> AFVVTDNCIKCKYC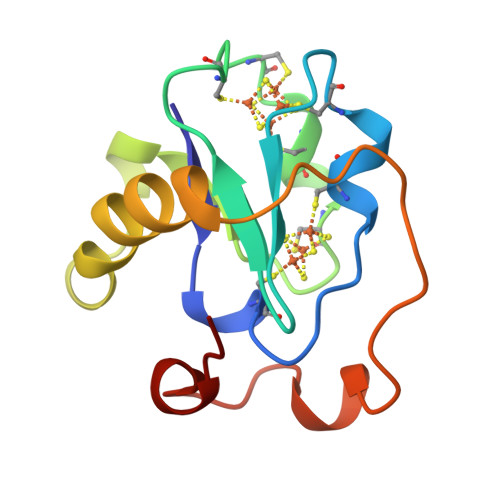DCVEVCPVDCFYEGPNFLVIHPDECIDCALCEPECPAQAIFSEDEVPEDMQEFIQLNAELAEVWPNITEKKDPLPDAEDWDGVKGKLQHLER> MASITQLFDDLCEALLPAAKTHLGQRSVNRKRAKRSLKKVAYNALFTNLFQDETQQLQPDMSKLPARNKILMLSFDLRVGGLGPKADRLEELVEELEAAPCCPLLEVGSVLDLLVQLAGSGPPQVLPRKRDYFLNNKHVGRNVPYSGYDCDDLSVFEMDVQSLISREECLCHSMIQETLQVMEAAPGTGLPTVGLFSFGDPCGDRFERDTRVSLFGALVHSRTYDMDVRLGLPPVPDNADLSGLAIKVPPSVDQWEDEGFQSASNLTPDSQSEPSVTPDVDLWEAALTYEASKRRCWERVGCPPGHREEPYLTEAGRDAFDKFCRLHQGELQLLAGGVLQAPQPVLVKECELVKDVLNVLIGVVSATFSLCQPAQAFVVKRGVHVSGASPESISSLLSEVAEYGTCYTRLSHFSLQPVLDSLYSKGLVFQAFTSGLRRYLQYYRACVLSTPPTLSLLTIGFLFKKLGRQLRYLAELCGVGAVLPGTCGGGPRAAFPTGVKLLSYLYQEALHNCSNEHYPVLLSLLKTSCEPYTRFIHDWVYSGVFRDAYGEFMIQVNHEYLSFRDKLYWTHGYVLISKEVEDCVPVFLKHIAHDIYVCGKTINLLKLCCPRHYLCWSDVPVPRISVIFSLEELKEIEKDCAVYVGRMERVARHSSVSKEEKELRMEIAKQELIAHAREAASRVLSALSDRQMSERMALDARKREQFQRLKEQFVKDQERRQAARQEELDDDFSYARELRDRERRLKSLEEELERKARQALVDHYSKLSAEAARREQKALWRIQRHRLESARLRFLLEDEKHIQEMLKAVSEAHQPQEPPDVLLSVHPQVTSPGPEHPEGGQGCDSGSAEQHSPAWDGWNRPGLLTPQPLKPLAVGAGGRGLQQAEGARPFSDSLSIGDFLPVGPGAEPSVQTGMVPLLEVALQTINLDLPPSAPGEAPAAASTQPSRPQEYDFSTVLRPAVATSPAPGPLQAAECSLGSSGLQLWEDSCGKMDACGSASRETLLPSHPPRRAALEEGSSQPTERLFGQVSGGGLPTGDYASEIAPTRPRWNTHGHVSDASIRVGENVSDVAPTQ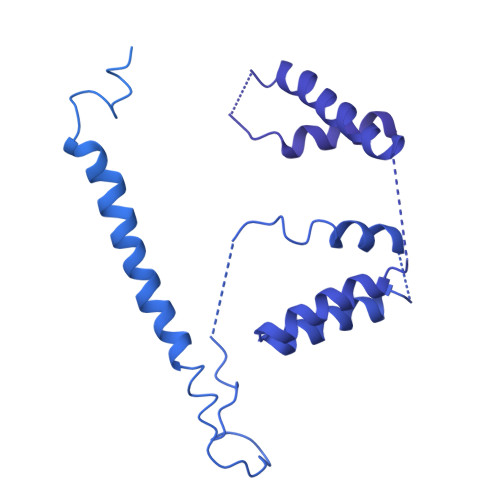PRWNTHGHVSNASISLGESVSDVAPTRPRWNIHGHVSNASIRVGENVSDVAPTRPRWNTHGHVSNASIRVGENVSDVAPTRPRWNTHGHVSDASISLGESVSDMAPARPRWNTHGHVSDASISLGESVSDMAPTRPRWNTHGHVSDTSIRVGENVSDVAPIRSRCNTHGHVSDASISLGEPVSDVVSTRPRWNTHVPIPPPHMVLGALSPEAEPNTPRPQQSPPGHTSQSALSLGAQSTVLDCGPRLPVEVGPSLSSPSSGCGEGSISVGENVSDVAPTQPWWPNTPGDSVSEELGPGRSGDTEDLSPNWPLNSQEDTAAQSSPGRGEEAEASAAEAQGGEQAYLAGLAGQYHLERYPDSYESMSEPPIAHLLRPVLPRAFAFPVDPQVQSAADETAVQLSELLTLPVLMKRSITAPLAAHISLVNKAAVDYFFVELHLEAHYEALRHFLLMEDGEFAQSLSDLLFEKLGAGQTPGELLNPLVLNSVLSKALQCSLHGDTPHASNLSLALKYLPEVFAPNAPDVLSCLELRYKVDWPLNIVITEGCVSKYSGVFSFLLQLKLMMWALKDVCFHLKRTALLSHMAGSVQFRQLQLFKHEMQHFVKVIQGYIANQILHVTWCEFRARLATVGDLEEIQRAHAEYLHKAVFRGLLTEKAAPVMNVIHSIFSLVLKFRSQLISQAWGPPGGPRGAEHPNFALMQQSYNTFKYYSHFLFKVVTKLVNRGYQPHLEDFLLRINFNNYYQDA>[3x]QDKITVTSEK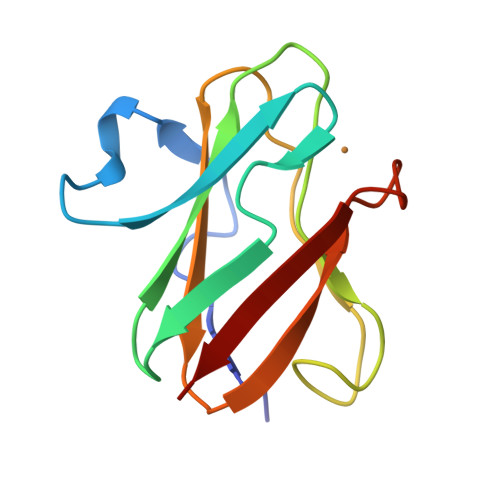PVAAADVPADAVVVGIEKMKYLTPEVTIKAGETVYWVNGEVMPHNVAFKKGIVGEDAFRGEMMTKDQAYAITFNEAGSYDYFCTPHPFMRGKVIVE4-(dimethylamino)-N-[7-(hydroxyamino)-7-oxoheptyl]benzamide | C16 H25 N3 O3 | 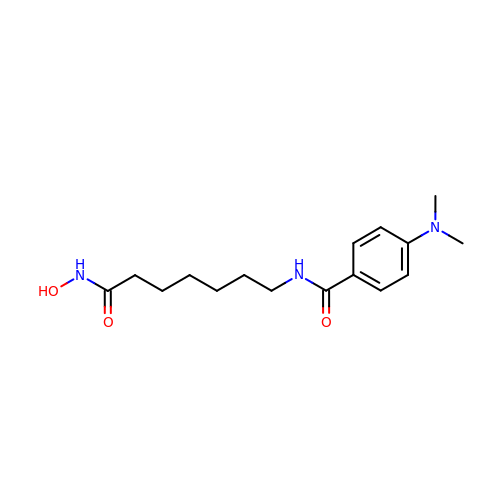MXWDSZWTBOCWBK-UHFFFAOYSA-N URACIL ARABINOSE-3'-PHOSPHATE 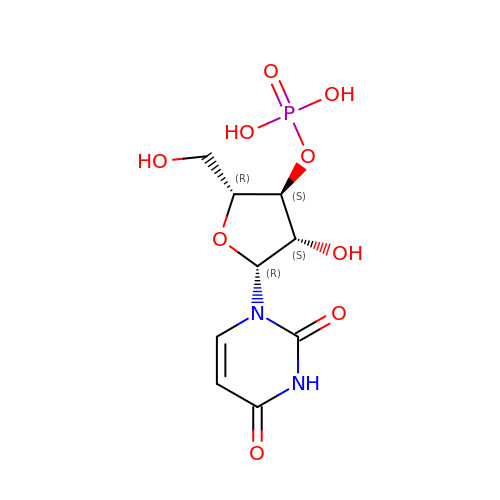| C9 H13 N2 O9 P | FOGRQMPFHUHIGU-PXBUCIJWSA-N> MVSLPRMVYPQPKVLTPCRKDVLVVTPWLAPIVW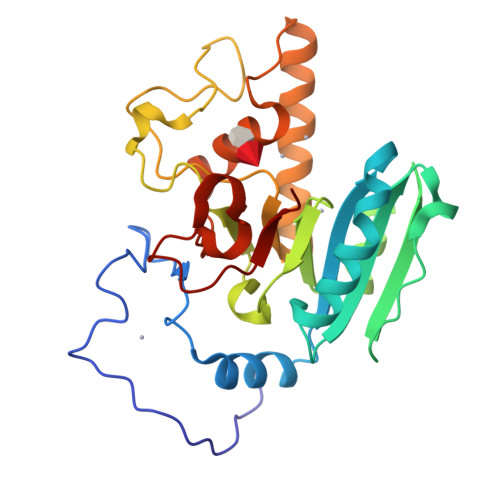EGTFNIDILNEQFRLQNTTIGLTVFAIKKYVAFLKLFLETAEKHFMVGHRVHYYVFTDQPAAVPRVTLGTGRQLSVLEVRAYKRWQDVSMRRMEMISDFCERRFLSEVDYLVCVDVDMEFRDHVGVEILTPLFGTLHPGFYGSSREAFTYERRPQSQAYIPKDEGDFYYLGGFFGGSVQEVQRLTRACHQAMMVDQANGIEAVWHDESHLNKYLLRHKPTKVLSPEYLWDQQLLGWPAVLRKLRFTAVP Phylogenetically diverse bacteria can carry out chloramphenicol reduction, but only a single enzyme has been described that efficiently catalyzes this reaction, the NfsB nitroreductase from Haemophilus influenzae strain KW20. We found that expression of H. influenzae and Neisseria spp. nfsB genes, but not Pasteurella multocida nfsB, allows Escherichia coli to resist chloramphenicol by nitroreduction. Mass spectrometric analysis confirmed that purified H. influenzae and N. meningitides NfsB enzymes reduce chloramphenicol to amino-chloramphenicol, while kinetics analyses supported the hypothesis that chloramphenicol reduction is a secondary activity. Previous kinetic studies of nitroreductase catalysis revealed that reactions progress by a double-displacement (ping-pong) mechanism that appears to lack the gating steps necessary to impose specificity, explaining the substrate promiscuity of these enzymes.

To understand better how variation in the substrate-binding site mediates activity, we solved the crystal structures of the NfsB homologs from Hi KW20, Hi Int1, Hi 86-028NP, and Nm Z2491. In contrast, Nm Z2491 NfsB was much less active in vitro, with ∼15% the activity as Hi KW20 NfsB (q < 0.0005), apparently driven by a much larger Km value. We found that the NfsB homologs studied here have Km values for chloramphenicol ranging from 160 µM for Hi 12 NfsB to 1,300 µM for Nm Z2491 NfsB, although all enzymes showed apparent kcat values near the median enzyme value of 13.7 s−1 (∼9 s−1 to ∼22 s−1). For example, the N. meningitidis NfsB enzyme has a comparatively low kcat/Km of ∼8 × 103 M−1 s−1 for chloramphenicol in vitro. When expressed in Es. coli, however, it confers an ∼8-fold increase in IC50 and an MIC double the clinical resistance cutoff of 8 µg/mL. For structural changes specific to substrate binding (e.g., nitroaromatics), as opposed to coenzyme binding (e.g., NADPH), we focused on comparisons between the Hi 12 NfsB structure complexed with 4-nitrophenol, the Nm Z2491 structure complexed with nicotinic acid, and the previously published En. cloacae structures complexed with 4-nitrobenzoic acid or NAAD. The phenyl rings of nicotinic acid in the Nm Z2491 NfsB structure and 4-nitrobenzoic acid in the En. cloacae structure coincide with the niacin ring of NAAD in the other En. cloacae structure. Intuitively, the Ser68-Met74 pair found in Hi 12 NfsB would provide more of the flexibility needed to properly locate and orient Trp71 to make space for the ribose of NADP than the Pro68-Ile74 pair in other H. influenzae NfsB homologs (Pro68-Ala74 in Nm Z2491 NfsB). Including the 4-nitrophenol-bound form of Hi 12 NfsB, the root mean square deviation (RMSD) of Cα atoms among these structures are very small with a range of 0.36 to 0.61 Å for the H. influenzae proteins and 0.9 Å for the Nm Z2491 structure.

>[4x]SNAMTVLDREQVLSAFKNRKSCRHYDAARKISAEDFQFILELGRLSPSSVGSEPWQFVVVQNPEIRQAIKPFSWGMADALDTASHLVVFLAKKNARFDSPFMLESLKRRGVTEPDAMAKSLARYQAFQADDIKILDDSRALFDWCCRQTYIALGNMMTGAAMAGIDSCPVEGFNYADMERVLSGQFGLFDAAEWGVSVAATFGYRVQEIATKARRPLEETVIWA Neplanocin-A | C11 H13 N5 O3 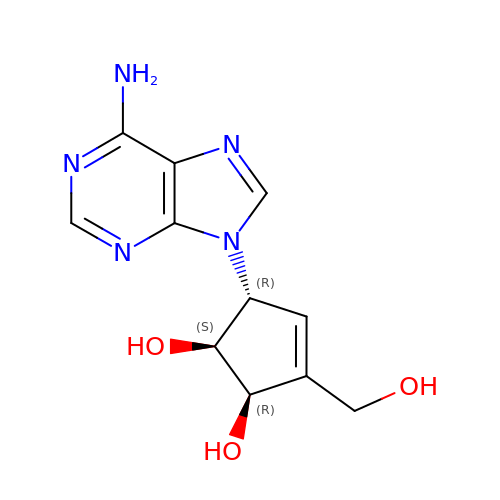| XUGWUUDOWNZAGW-VDAHYXPESA-N(2~{S})-4-(cyclobutylmethyl)-2-(2,4-dichlorophenyl)-~{N}-(2-methylpropylsulfonyl)-2,3-dihydro-1,4-benzoxazine-6-carboxamide 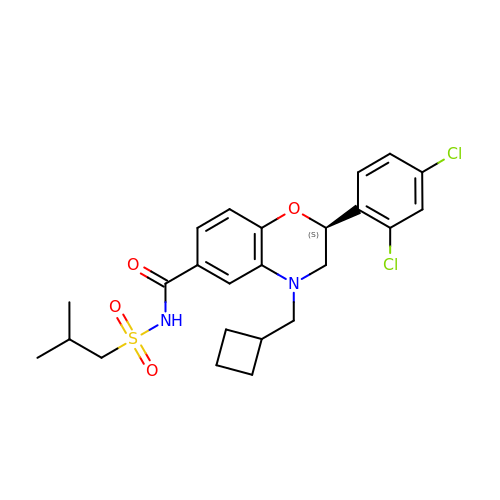| C24 H28 Cl2 N2 O4 S | UHSJMFUMFQAOOO-HSZRJFAPSA-N>[2x]HHHHHHAFLEDGSARLEARTVYFNRDFRDGSSANPQGASKREEAAQGFILDLRSGYTEGALGFGVDTL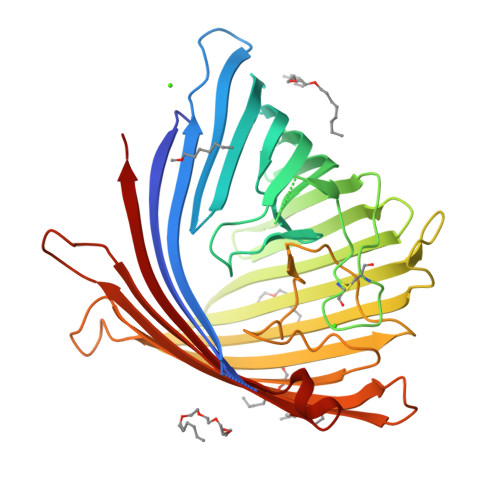AMLGIKLDSSPADSNSGLLPSSGHDPRRSVDQYAKAGVAGKMRFSQTQFRYGAMLPDMPLLKYNDGRLLPTLFHGAQLTSEEIAGLRFSATRLERYTARDSSDAQDIRLHCKNKRYACDTTGNRFDAYQLDYQVNDGLLLQYAQGGLRNVYRQRYLGAVGKRQVGAGKLSADLRWFDSEDAGAARAGKIDNRALSLLLAYAQGGHTLSAGWQRMNGASSMPYLDGSNPYLANYLQVNDFANPEERSWQLRYDFDLRSVGVPGLSFMTRYVNGDHIRLANGDEGKEWERDIELKYIVQSGRFKDLSLRLRNATYRTDFERSARDVDEVRLIASYNLSLF(7R,12R,13R)-13-formyl-12,14-dihydroxy-3,5,7-trimethyltetradeca-2,4-dienoic acid | C18 H30 O5 | 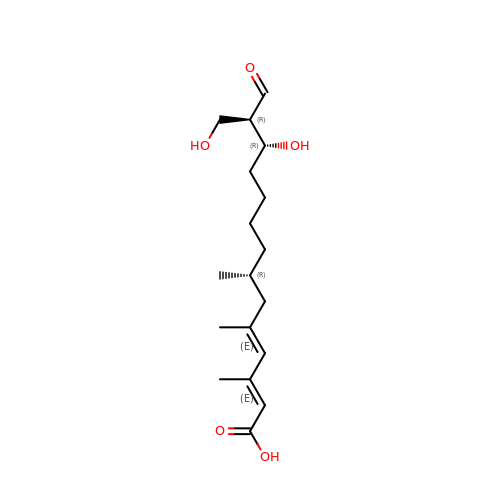CJCDMTWCUXKYGF-QPILVHKNSA-N Hydrogen disulfide | 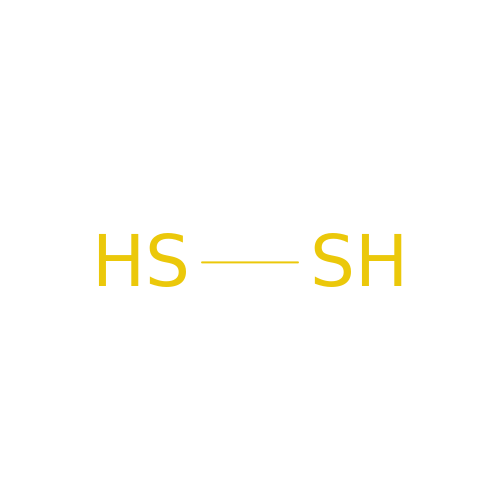H2 S2 | BWGNESOTFCXPMA-UHFFFAOYSA-N2-azanyl-5-chloranyl-benzamide | C7 H7 Cl N2 O | 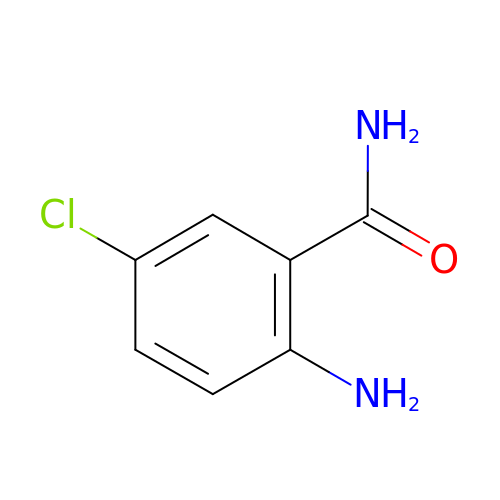DNRVZOZGQHHDAT-UHFFFAOYSA-N>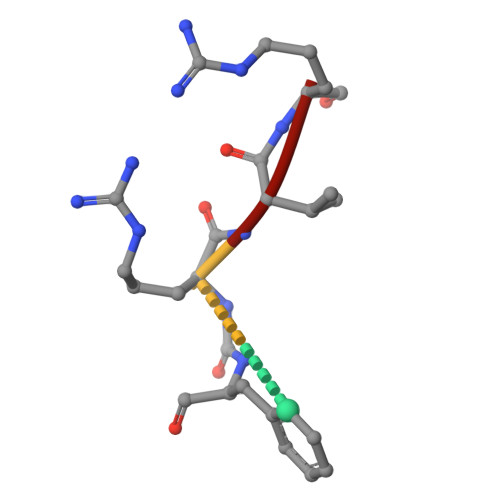 FRVR> GSTAEKNRKDAEEWFFTKTEELNREVATNSELVQSGKSEISELRRTMQNLEIELQSQLSMKASLENSLEETKGRYCMQLAQIQEMIGSVEEQLAQLRCEMEQQNQEYKILLDVKTRLEQEIATYRRLLEGE;> MANRSRTEAESWYQTKYEELQQTAGRHGDDLRNTKHEISEMNRMIQRLRAEIDNVKKQCANLQNAIADAEQRGELALKDARN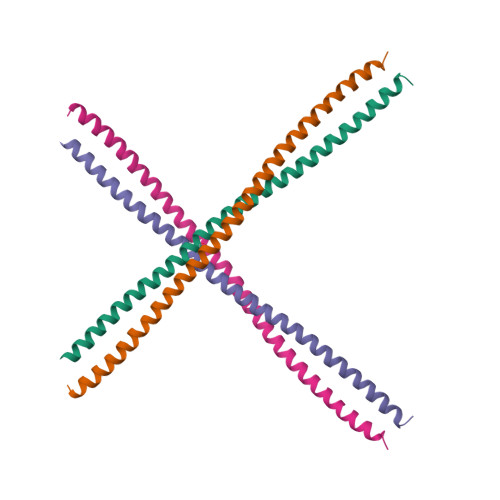KLAELEEALQKAKQDMARLLREYQELMNTKLALDVEIATYRKLLEGE> GEFTQSVSRLQSIVAGLKNAPSDQLINIFESCVRNPVENIMKILKGIGETFCQHYTQSTDEQPGSHIDFAVNRLKLAEILYYKILETVMVQETRRLHGMDMSVLLEQDIFHRSLMACCLEIVLFAYSSPRTFPWIIEVLNLQPFYFYKVIEVVIRSEEGLSRDMVKHLNSIEEQILESLAWSHDSALWEALQVSANKVPTCEEVIFPNNFETGNNRPKRTGSLALFYRKVYHLASVRLRDLCLKLDVSNELRRKIWTCFEFTLVHCPDLMKDRHLDQLLLCAFYIMAKVTKEERTFQEIMKSYRNQPQANSHVYRSVLLKSIKEERGDLIKFYNTIYVGRVKSFALKYDLANQDHMMDAPPLSPFPHIKQQ;>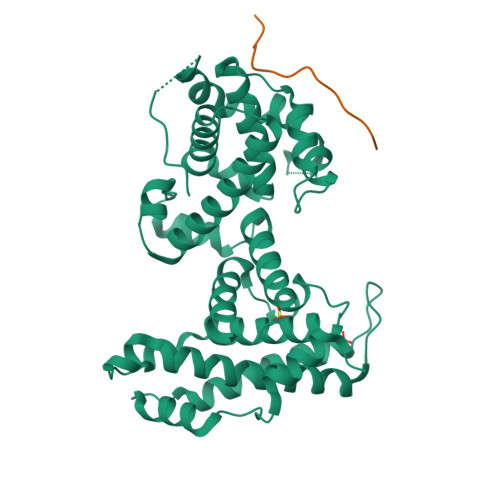 LTEELGCDEIIDRE> GPGKRVYQIGSSSRDVQVCPRGAGAALRQEIEDKQLMVNNLTDELQDAIDEANPAEIANTSQQLRHARADLADLQRRFAVLRNEDRRINQ;> SESKVKKVVSIPAIDEGDLWTWRKYGQKDILGSRFPR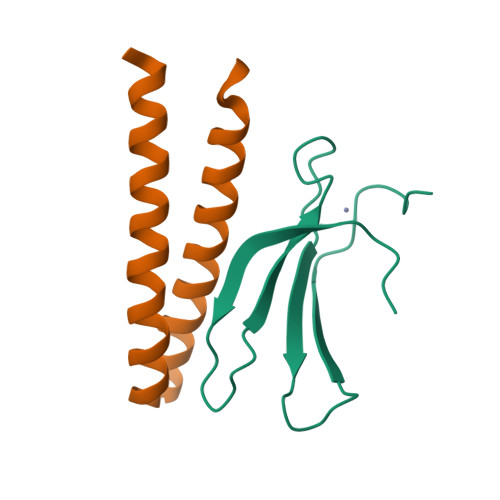GYYRCAYKFTHGCKATKQVQRSETDSNMLAITYLSEHNHPRPT>SRVENSNGQSQPAATSKTVKDNAEIYYDDDDSDRFYFHVWGGEDIHVGLYKEPVDQDEIREASLRTDEWLASELAMTGVLQRQAKGLDLGAGYGGAARFLVRKFGVSIDCLNIAPVQNKRNEEYNNQAGLADNITVKYGSFLEIPCEDNSYDFIWSQDAFLHSPDKLKVFQECARVLKPRGVMAITDPMKEDGIDKSSIQPILDRIKLHDMGSLGLYRSLAKECGLVTLRTFSRPDSLVHHYSKVKAELIKRSSEIASFCSPEFQANMKRGL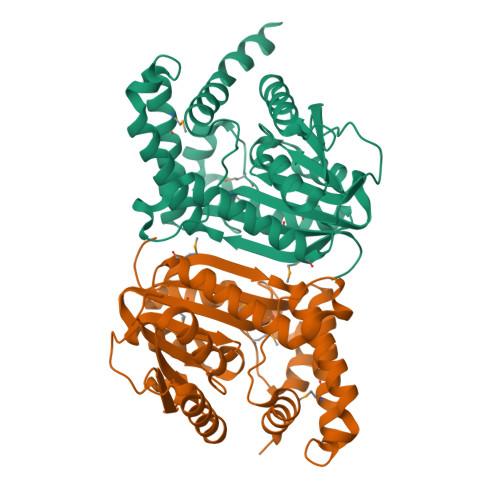EHWIEGGRAGKLTWGGMLFRKSDKI[4x]The iron-dependent regulator IdeR is the main transcriptional regulator controlling iron homeostasis genes in Actinobacteria, including species from the Corynebacterium, Mycobacterium and Streptomyces genera, as well as the erythromycin-producing bacterium Saccharopolyspora erythraea. IdeR is an OCS from the DtxR (Diphtheria toxin repressor) family of transcriptional regulators which typically consist of three domains: an N-terminal DNA-binding winged helix-turn-helix (wHTH) motif, followed by a dimerization interface that contains most of the metal-binding residues, and a C-terminal SH3-like domain (21–23). The main function of IdeR is to repress the expression of iron uptake genes when the intracellular iron levels are sufficient. When iron levels are sufficient for iron ions to occupy the IdeR metal-binding sites, the regulator is activated and recognizes a highly conserved 19-bp sequence located in the promoter region of its target genes.

Due to the similarities between both metals, and the constraints of working with Fe2+, we used Co2+ to activate IdeR in all of the subsequent DNA-binding experiments. We then co-crystallized IdeR with a 30-bp double-stranded DNA oligomer containing the consensus sequence TTAGGTTAGSCTAACCTAA (S = G or C, i.e. G in the forward strand and C in the reverse strand). Crystal structures were obtained for the complexes with the physiological activator Fe2+ as well as the mimic Co2+. Both crystallized in space group C2, containing four polypeptide chains forming two dimers and two DNA strands forming a distorted B-type double helix in the asymmetric unit. Each IdeR subunit binds to one of the four CCTAA repeats of the recognition sequence, one dimer interacting with repeats 1 and 3 and the other with repeats 2 and 4. Both metal-binding sites of each IdeR subunit are occupied in both the Fe2+ and Co2+ complexes. No significant differences between the Fe2+-activated and Co2+-activated IdeR-DNA complexes can be discerned, neither globally, nor at the metal-binding sites. The structures of these IdeR dimers are very similar to the DNA-free dimer structure. Notably, only one direct hydrogen bond is formed between the protein and a DNA base, between Gln43 and the first cytosine of each CCTAA repeat, or guanine at the central G-C basepair of the palindrome. Interestingly, in the DNA complex structures we observe a swap of the SH3-like domains of one subunit of each IdeR dimer with a symmetry-related chain.

>GHMNDLIDTTEMYLRTIYDLEEEGVVPLRARIAERLEQSGPTVSQTVARMERDGLLTVAEDRHLELTKAGRARAISVMRKHRLAERLLVDVIGLEWEQVHLEACRWEHVMSEAVERKLVKLLGNPTTSPYGNPIPGLDELGVGDSVEPVDTDLRRVDEVARSGGGRALVCRIAEHVQLDPDLMSELKKVGVVPGNEIDIVAVAGVNKPIQVQGSEGGTQLQPGIAHAVMVRVK[6x]>[6x]MDRSLRPEEIEELREAFREFDKDKDGYINCRDLGNCMRTMGYMPTEMELIELSQQINM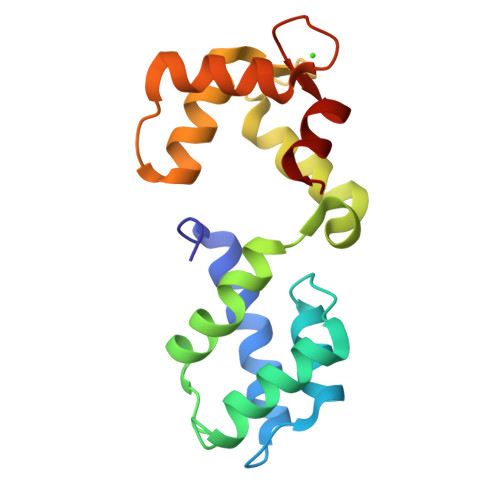NLGGHVDFDDFVELMGPKLLAETADMIGVKELRDAFREFDTNGDGEISTSELREAMRKLLGHQVGHRDIEEIIRDVDLNGDGRVDFEEFVRMMSR>GSGETKVIYHLDEEETPYLVKIPVPAERITLGDFKSVLQRPAGAKYFFKSMDQDFGVVKEEISDDNARLPCFNGRVVSWLVSS[12x]

A current model for signal transduction is that ligand-bound Fzd recruits the cytosolic protein Dishevelled (Dvl), which then binds to Axin and thereby recruits the destruction complex to the activated receptor complex. The Dvl-Axin interaction is essential for Wnt/β-catenin signal transduction and is mediated by a DIX (Dvl and Axin interacting) domain present in each protein. Dvl has an N-terminal DIX domain, as well as a PDZ and a DEP domain; the DEP domain mediates the interaction with Fzd. We found that purified Dvl DIX in solution forms antiparallel, double-stranded filaments whose stability depends on the inter-strand interactions in the double helix.

We obtained a cryo-electron microscopy (cryo-EM) map of the DIX filaments with a global resolution of 3.6 Å, which enabled a near atomic resolution structure. Remarkably, unlike the single stranded fibers observed in crystals of Dvl2 DIX domains, in solution the Dvl2 DIX filament forms an antiparallel double helix. Successive protomers in the filament are related by a rotation of 48.0 ± 0.2° around the helical axis, with a rise of 13.5 ± 0.3 Å per protomer. The pitch of the helix is 101.3 Å, larger than the pitch of the single stranded helix observed in crystals of Dvl2 Y27D (85 Å) and Y27W/C80S (88 Å). The head-to-tail interface within each strand is similar to that observed in crystal structures. For example, Y27 packs against F56 and K68 of a neighboring protomer. We next tested the role of the inter-strand contacts that form the antiparallel double helix. These contacts are formed between two opposing protomers, principally by the β3-β4 (residues 60–66) and β4-β5 (residues 82–84) loops. Some residues on the β3-β4 loop (e.g., D63) participate in intra- and inter-strand interactions, whereas others appear to be involved solely in inter-strand contacts, including M60, G65 and N82. The structural, biochemical and signaling data indicate that the double stranded DIX filament is stabilized by inter-strand, antiparallel contacts that are functionally important.>GSENKKIMLESAMTLRNITNIKTHSPVELLNEGKIRLEDPMDFESQLIYPALIMYPTQDEFDFVGEVSELTTVQELVDLVLEGPQERFKKEGKENFTPKKVLVFMETKAGGLIKAGKKLTFHDILKKESPDVPLFDNALKIYIVPKVESEGWISK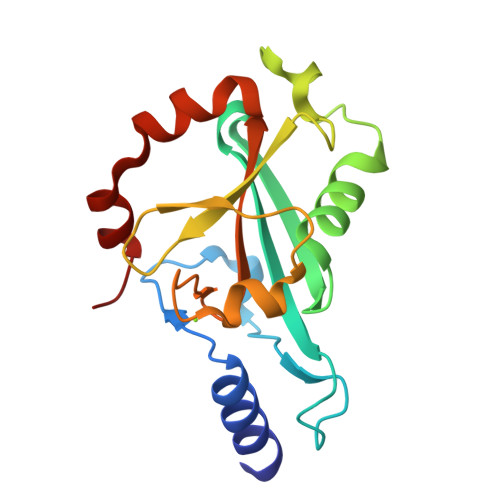WDKQKALERRSV[2x]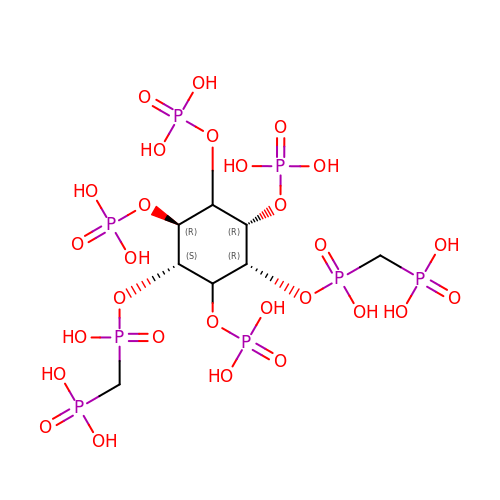3,5-di-methylenebisphosphonate inositol tetrakisphosphate | C8 H24 O28 P8 | WDYISGXURTYYJP-XAZAIFFQSA-N>[2x]MGIQLLDKYQLQPLSLDSVPWRRQPGQQVLWIGCSDSGADELESSGLPADEIFEYRSLGNMMVDDLSCKATLGYALDSLKIRNIVICGHYGCHIASGEVNAGLQKPWSSVLDTLRST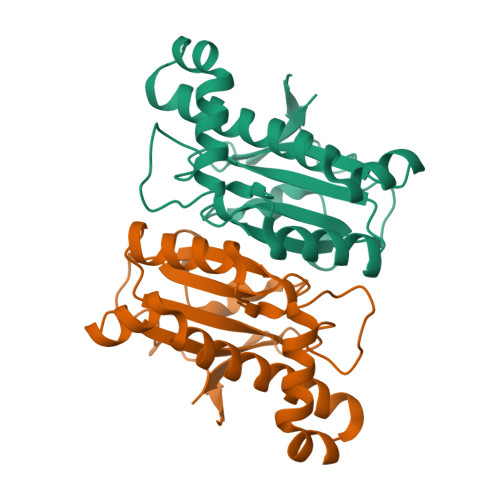HRRTLDSLTGTERDRALVELNVLEQVHSLRQSAEAAEALQKQQLNIWGMVYDKATKRGYQLIEA>MLCALSGEIPEEPVVSKKTGVLFEKRLILKYLEEHNNIEPGTTEEL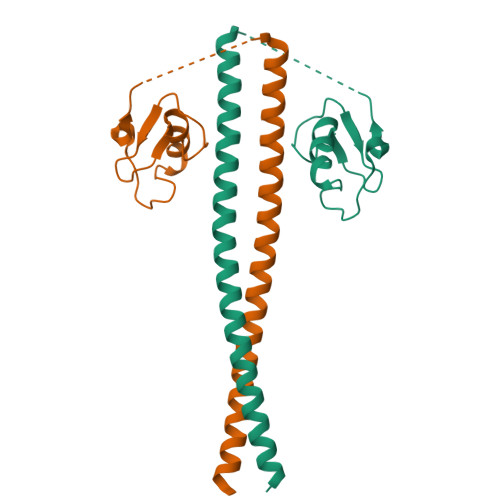DPETDLLPIKTSRVVRPRPPNFTSIPSLLKAFQDEWDALVLETYTTREQLARVREELATALYQHDAAVRVIARLTRERDEAREALARLTV[2x]>[2x]MITTSPRHRRARRVVSLLTTAGLVATAAVALAAPAHAGTTLGQSAAERGRYFGVAIAAGR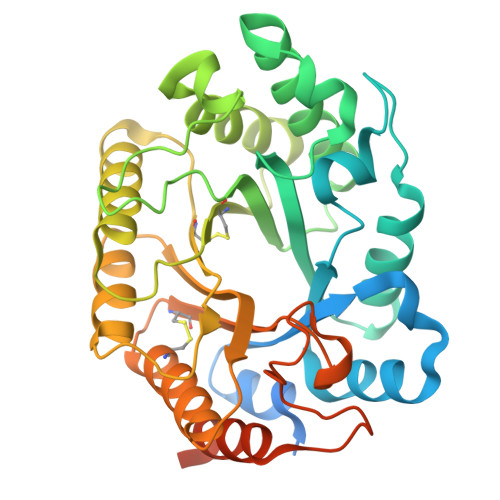MNDGTYMGIVDREFDSIVAENEMKMDATEPNRNQFNFSNGDRIVNYALGKGKKVRGHTLAWHAQQPGWMQNMSGQSLRDALLNHVSRVASYYRGKIHSWDVVNEAFADDGRGSRRDSNLQRTGNDWIEAAFRAARSADPGAKLCYNDYNTDGVNAKSTGVYNMVRDFKARGVPIDCVGFQSHLGTTVPSDYQANLQRFADLGVDVQITELDIQQGSNQANAYRQVVQACLAVSRCTGITVWGVRDTDSWRTGANPLLFDGSGNKKAAYAAVLEALNAGGGNGGGNNGGGSSSVDTNAWYV>GAAGGUUUUUCUUUUUCCUGAAGGCGAAAGUCUUCAGGUUUUUCUUUUUGGCCUUUCUUAAAAAAAA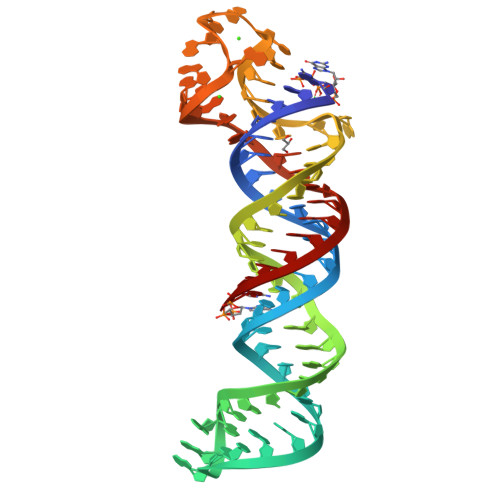AAAAAGAAAA[2x]>[3x]MKIGDISIHYLNGGNTKMDGGAMFGVVPKPLWSKQYNANERNQINLPTHPILIQTAQYNLIIDAGIGNGKLSEKQLRNFGVDEESHIIADLANYNLTPKDIDYVLMTHMHFDHAAGLTDQAGHAIFENAIHVVQQDEWHEFIAPNIRSKSTYWDKNKGDYSNKLILFEKHFEPVPGIKMQHSGGHSFGHTIITIESQGDKAVHMG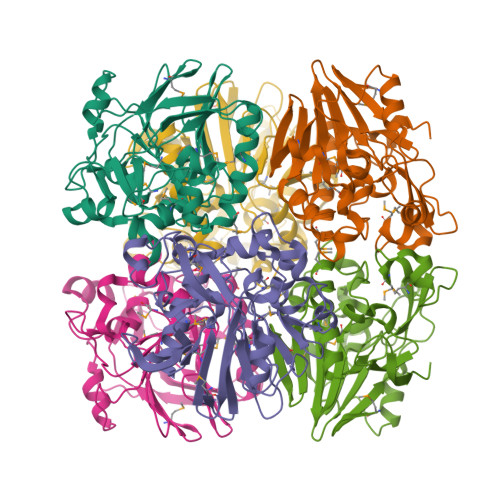DIFPTTAHKNPLWVTAYDDYPMQSIREKERMIPYFIQQQYWFLFYHDENYFAVKYSDDGENIDAYILRETLVDNN> MIVSAIAANALLESVTKFHCGVIYDYSTAEYVSYRPSDFGAYLDALEAEVARGGLIVFHNGHKYDVPALTKLAKLQLNREFHLPRENCIDTLVLS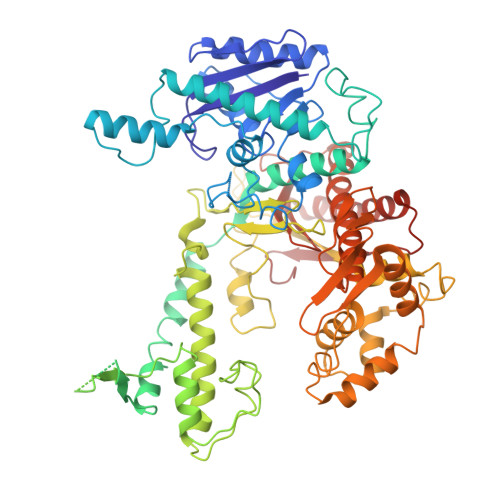RLIHSNLKDTDMGLLRSGKLPGKRFGSHALEAWGYRLGEMKGEYKDDFKRMLEEQGEEYVDGMEWWNFNEEMMDYNVQDVVVTKALLEKLLSDKHYFPPEIDFTDVGYTTFWSESLEAVDIEHRAAWLLAKQERNGFPFDTKAIEELYVELAARRSELLRKLTETFGSWYQPKGGTEMFCHPRTGKPLPKYPRIKTPKVGGIFKKPKNKAQREGREPCELDTREYVAGAPYTPVEHVVFNPSSRDHIQKKLQEAGWVPTKYTDKGAPVVDDEVLEGVRVDDPEKQAAIDLIKEYLMIQKRIGQSAEGDKAWLRYVAEDGKIHGSVNPNGAVTGRATHAFPNLAQIPGVRSPYGEQCRAAFGAEHHLDGITGKPWVQAGIDASGLELRCLAHFMARFDNGEYAHEILNGDIHTKNQIAAELPTRDNAKTFIYGFLYGAGDEKIGQIVGAGKERGKELKKKFLENTPAIAALRESIQQTLVESSQWVAGEQQVKWKRRWIKGLDGRKVHVRSPHAALNTLLQSAGALICKLWIIKTEEMLVEKGLKHGWDGDFAYMAWVHDEIQVGCRTEEIAQVVIETAQEAMRWVGDHWNFRCLLDTEGKMGPNWAICH> MRVLGIETSCDETGIA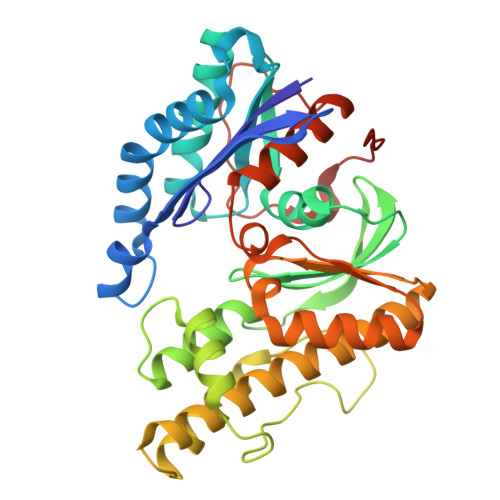IYDDEKGLLANQLYSQVKLHADYGGVVPELASRDHVRKTVPLIQAALKESGLTAKDIDAVAYTAGPGLVGALLVGATVGRSLAFAWDVPAIPVHHMEGHLLAPMLEDNPPEFPFVALLVSGGHTQLISVTGIGQYELLGESIDDAAGEAFDKTAKLLGLDYPGGPLLSKMAAQGTAGRFVFPRPMTDRPGLDFSFSGLKTFAANTIRDNGTDDQTRADIARAFEDAVVDTLMIKCKRALDQTGFKRLVMAGGVSANRTLRAKLAEMMKKRRGEVFYARPEFCTDNGAMIAYAGMVRFKAGATADLGVSVRPRWPLAELPAAHHHHHH> MSAMNARQGILSLALKDKAALYSAYMPFVKSGGIFVPTPKRYMLGDEVFLLLTLPDSSERLPVAGKVVWTTPAGAQGNRAAGIGVQFPDGPE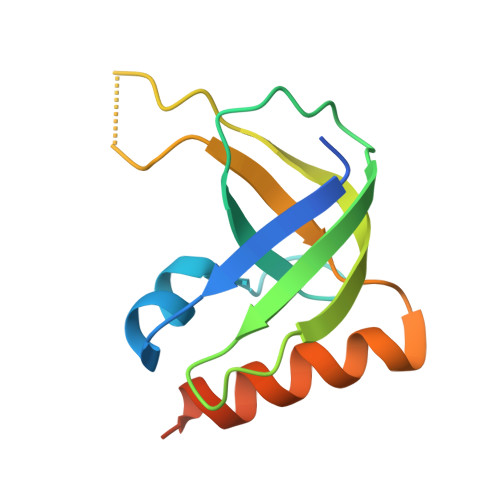GEAVRNKIETLLAGLTTSDKPTHTM> FQG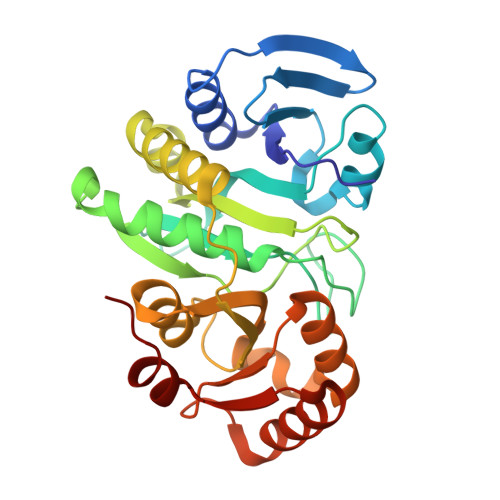HMKLVVCSESDTAGQNIKDNLLTFADFEEKDVGEFKLYLSDEFYIAETKERLIYADHIDEKLAKYIDFEEILFASRHSSKDGRKIFTVHVSGNVGTADFGGKPYSLAKPSPQTMKNYVLALRERLDRKPEFEFTMEVTHHGPSEISKPSAFYEIGSTEEEWKDREAAEVVAEAMLDAIRAEKMDWNVAVGVGGTHYAPRQTEIMLTTTFTFGHNFAKYTFEHLTAEFLVKAVKLSEAEYIIIDEKSVNSAVKKIVNEAAEVAGVEVLKSKKVKKDFRLV> ESTEFEKNQKRYQDLISTFPHEKGWRPKEPLIEYGGYWWLPSLLEGCIHAQEFFQARPSDFLVCSYPKTGTTWLKALTFAIANRSRFDDSSNPLLKRNPHEFVPYIEIDFPFFPEVDVLKDKGNTLFSTHIPYELLPDSVVKSGCKMVYIWREPKDTFISMWTFLHKERTELGPVSNLEESFDMFCRGLSGYGPYLNHILAYWKAYQENPDRILFLKYETMRADPLPYVKSLAEFMGHGFTAEEEEKGVVEKVVNLCSFETLKNLEANKGEKDREDRPGVYANSAYFRKGKVGDWSNYLTPEMAARIDGLMEEKFKGTGLLE

Sulphotransferases (SOTs or SULTs) (EC 2.8.2.-) can be found in all organisms analysed so far. They catalyse the transfer of a sulfuryl group from the co-substrate 3′-phospho- adenosine 5′-phosphosulphate (PAPS) to a hydroxyl group of various substrates. Here we report crystal structures of the AtSOT18 binary complex with PAP and a ternary complex with PAP and sinigrin.

Several atomic positions occupied by the polar groups of sinigrin in the AtSOT18•PAP•sinigrin complex, including the sulphate moiety, are filled with solvent molecules in the AtSOT18•PAP complex structure. In the AtSOT18•PAP complex, the main conformation of Met186 is oriented away from the acceptor site. Our mutagenesis study showed that the disturbance of these interactions leads to a dramatic loss of enzymatic activity. This seeming contradiction is resolved by our AtSOT18•PAP complex structure, where the oxygen positions of the sulphate moiety are occupied by the oxygen atoms of ethylene glycol. The solvent oxygens in AtSOT18•PAP complex occupying the place of the sulfuryl group in the AtSOT18•PAP•sinigrin complex are very stable and have excellent electron density and low B-factors. The necessity to replace solvent oxygen atoms upon binding of the sulfuryl group leads to a near zero binding enthalpy balance, which explains the results of experimental kinetics analysis. The main contribution to the PAPS binding energy is thus provided by the PAP nucleotide moiety, which binds to a deep hydrophobic pocket between helices α3, α13 and α16, and the 3′-phosphate group. PAP is deeply embedded within the structure and stabilized by several hydrogen bonds and π-π stacking with surrounding amino acids. The four oxygen atoms of the 3′-phosphate group form six hydrogen bonds with the side chains of Arg177, Ser185, Arg313, and the main chain of Lys314 and Gly315. The oxygen atoms of the 5′-phosphate group make six hydrogen bonds to the side chains of Lys93, the main chain of Gly95, and both the main and the side chains of Thr96 and Thr97. The adenyl moiety of PAP is stabilized by hydrogen bonds with Cys282 and Tyr243, the stacking interaction with Trp98, and the hydrophobic contacts with Phe284 and aliphatic groups of Arg247.>GQDAKESEVRKVDAFSSIEITSVGTIHFTQSDTYSFRIEGREKYVKNTETTVKDGRLLIGFKDKKNKSRRNQKDGVTIWISAPDLKEVEFTGVGEFNCEKPLKLDEVSFEVKGVGEVNVADLTCNVLKVALRGVGSADIHVVCDYLSAQMGGVGSVTLSGSAGRADISKGGIGGVNTDNLKIGR[4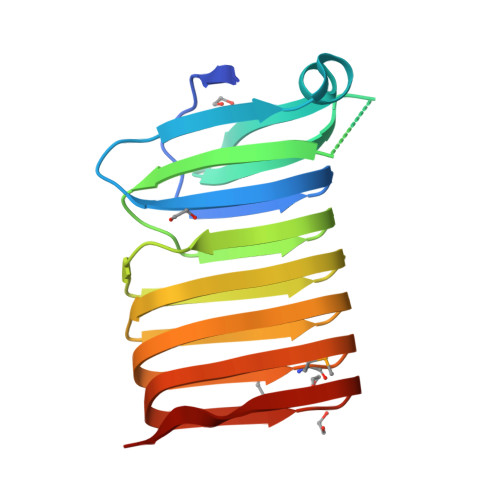x]> GSMAEDWLDCPALGPGWKRREVFRKSGATCGRSDTYYQSPTGDRIRS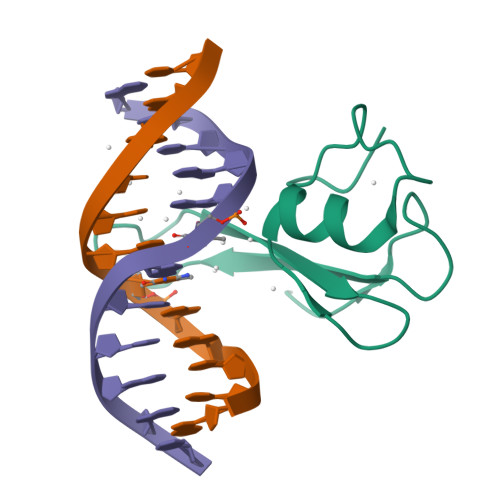KVELTRYLGPACDLTLFDFKQGILCYPAPKAH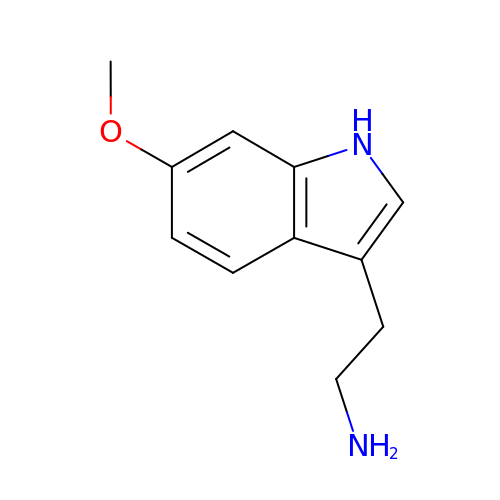2-(6-methoxy-1H-indol-3-yl)ethanamine | C11 H14 N2 O | VOCGEKMEZOPDFP-UHFFFAOYSA-N2,1,3-benzothiadiazol-4-ylmethanamine | C7 H7 N3 S | 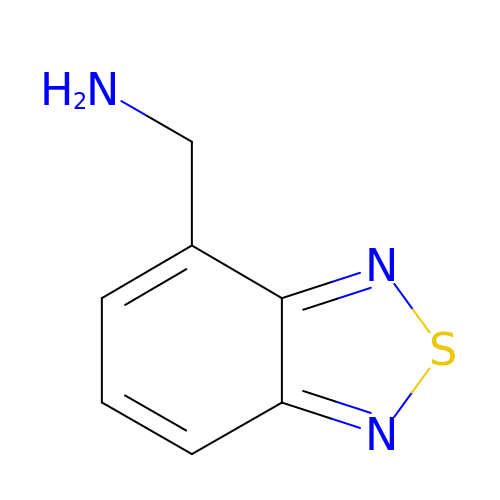HMEXAOROCQLCJX-UHFFFAOYSA-N>[6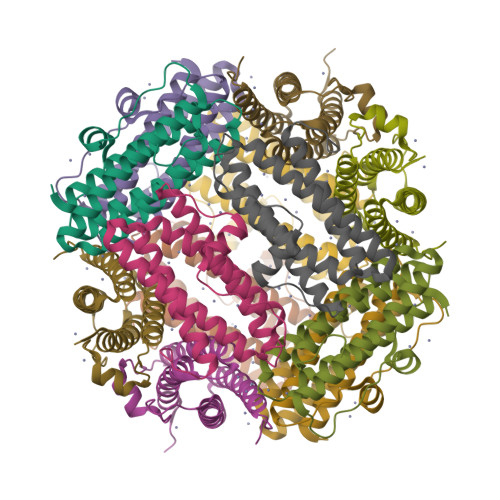x]MKTINSVDTKEFLNHQVANLNVFTVKIHQIHWYMRGHNFFTLHEKMDDLYSEFGEQMDEVAERLLAIGGSPFSTLKEFLENASVEEAPYTKPKTMDQLMEDLVGTLELLRDEYKQGIELTDKEGDDVTNDMLIAFKASIDKHIWMFKAFLGKAPLE3-ethoxy-~{N}-(2-methyl-1,2,3,4-tetrazol-5-yl)benzamide 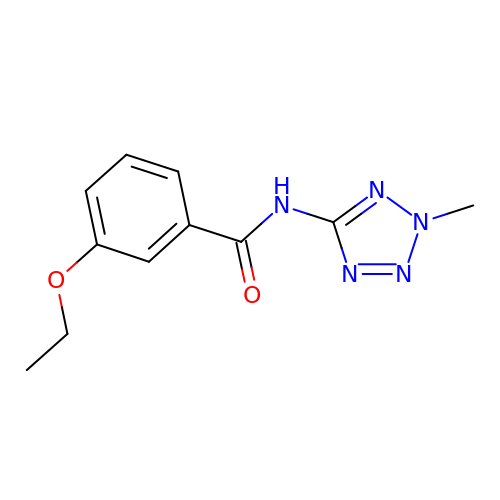| C11 H13 N5 O2 | QUQSTKZNAZQZRQ-UHFFFAOYSA-N> MAHHHHHHMSNSAMSVVILAAGKGTRMYSDLPKVLHTLAGKPMVQHVIDAAKDLGAAAVHLVYGHGGDLLRQTLHEDNLNWVLQAEQLGTGHAMQQAAPFFSDDEDILMLYGDVPLISVETLQRLRAAKPQGGIGLLTVKLDDPTGYGRITRENGQVTGIVEHKDASEAQRQIQEINTGILVANGADLKRWLAKLTNNNAQGEYYITDIIAMAYQEGHEIVAVHPQRLSEVEGVNNRLQLARLERVYQSEQAEKLLLAGVMLRDPARFDLRGVLKHGRDV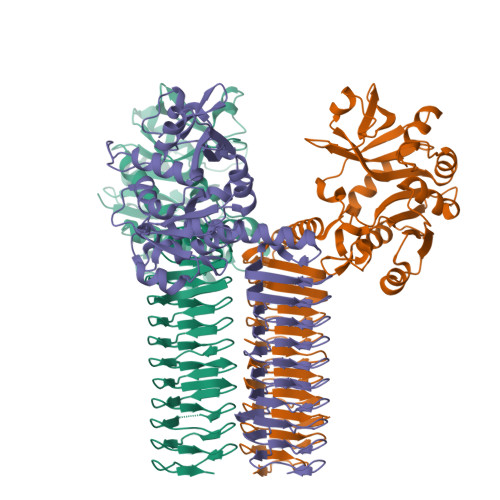EIDTNVILQGHVVLGDRVKIGAGCVIKDSVIGDDCEISPYSVVEDAQLQAACTIGPFARLRPGAELLEGAHVGNFVEMKKARLGKGSKAGHLSYLGDAEIGDNVNIGAGTITCNYDGANKHKTIIGDDVFVGSDTQLVAPVSVGNGVTIAAGTTVTRNIADNELVLSRVPQVHKQGWQRPVKKK> IVGGYTCGANTVPYQVSLNSGYHFCGGSLINSQWVVSAAHCYKSGIQVR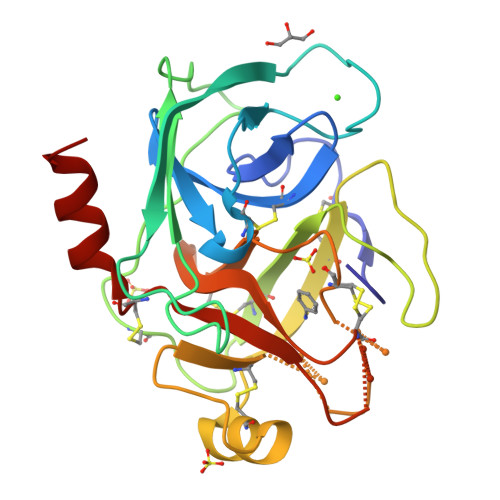LGEDNINVVEGNEQFISASKSIVHPSYNSNTLNNDIMLIKLKSAASLNSRVASISLPTSCASAGTQCLISGWGNTKSSGTSYPDVLKCLKAPILSDSSCKSAYPGQITSNMFCAYGLEGKGDSCQGDSGGPVVCSGKLQGIVSWGSGCQAKNKPGVYTKVCNYVSWIKQTIASN>SEVGNSQAVCPGTLNGLSVTGDAENQYQTLYKLYERCEVVMGNLEIVLTGHNADLSFLQWIREVTGYVLVAMNEFSTLPLPNLRVVRGTQVYDGKFAIFVMLNYNTNSSHALRQLRLTQLTEILSGGVYIEKNDKLCHMDTIDWRDIVRDRDAEIVVKDNGRSCPPCHEVCKGRCWGPGSEDCQTLTKTICAPQCNGHCFGPNPNQCCHDECAGGCSGPQDTDCFACRHFNDSGACVPRCPQPLVYNKLTFQLEPNPHTKYQYGGVCVASCPHNFVVDQTSCVRACPPDKMEVDKNGLKMCEPCGGLCPKACEGTGSGSRFQTVDSSNIDGFVNCTKILGNLDFLITGLNGDPWHKIPALDPEKLNVFRTVREITGYLNIQSWPPHMHNFSVFSNLTTIGGRSLYNRGFSLLIMKNLQVTSLGFRSLKEISAGRIYISANRQLCYHHSLNWTKVLRGPTEERLDIKHNRPRRDCVAEGKVCDPLCSSGGCWGPGPGQCLSCRNYSRGGVCVTHCNFLNGEPREFAHEAECFSCHPECQPMEGTATCNGSGSDTCAQCAHFRDGPHCVSS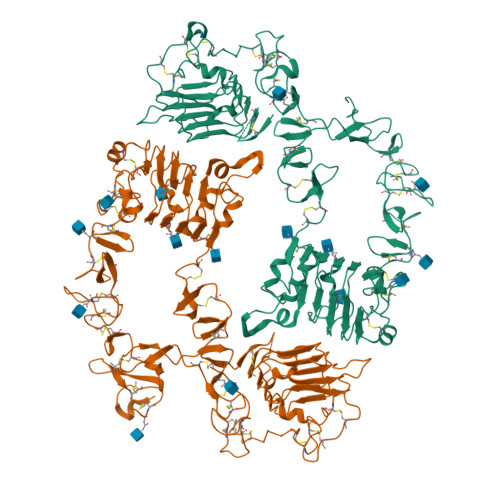CPHGVLGAKGPIYKYPDVQNECRPCHENCTQGCKGPELQDCLGQTLVLIGK[2x]>[4x]SNAMDILRKGNKDLIKDINRYTVLNLIREKGEITRTEIAKKCDFGMSTLTYILDDLQQEGIILEGAETSSTGGRRAKLVRFNKDYGFVVSVKVEEEQLLFALTDLNAEIIENTSIPFSSEKKPEEAIELIAKNVKKMCGNRDMNHLLGVGIAISGLVNRKKGTVIRSTMLGWENVALEAMLHAHFPDIPVYVDKNINCYTLAELWLGEG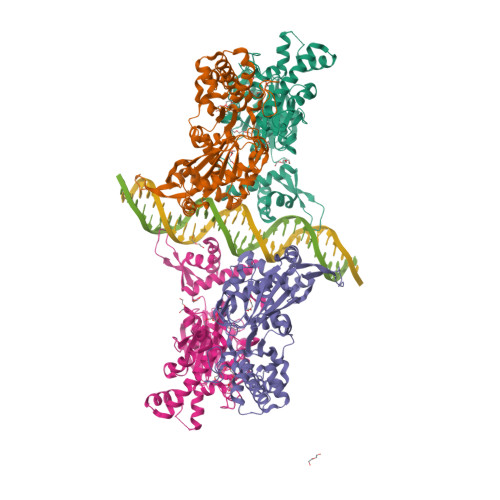KQSNNFATVSVGAGLGLSVVINRQIYYGAQGGAGEFGHTTIQPGGYKCHCGQKGCLEMYASEFYFRNRGEELKEAYPTSELNDFHFDKVAKSARAGDEMATELMGKMGEYLGYGIRNIINTFNPEKVIIVGEGLHHRDLFLTKIDEIASQNFFSGAGFETEITTTSLEDPAWLQGAALLVIHQLFQVPIYEEEQTLLR>[2x]MSAPKPFVIGIAGGTASGKTTLAQALARTLGERVALLPMDHYYKDLGHLPLEERLRVNYDHPDAFDLALYLEHAQAL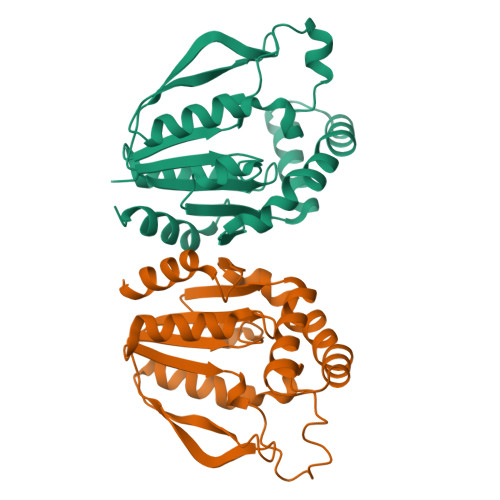LRGLPVEMPVYDFRAYTRSPRRTPVRPAPVVILEGILVLYPKELRDLMDLKVFVDADADERFIRRLKRDVLERGRSLEGVVAQYLEQVKPMHLHFVEPTKRYADVIVPRGGQNPVALEMLAAKALARLARMGAA>MKSVITTTISAADAAGRYPSTSDLQSVQGNIQRAAARLEAAEKLGSNH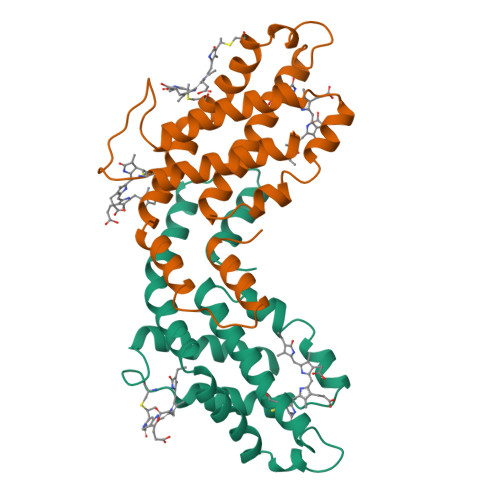EAVVKEAGDACFSKYGYNKNPGEAGENQEKINKCYRDIDHYMRLINYTLVVGGTGPLDEWGIAGAREVYRTLNLPSAAYIAAFVFTRDRLCIPRDMSAQAGVEFCTALDYLINSLS[2x];>[2x]MLDAFSRVVVNSDSKAAYVSGSDLQALKTFINDGNKRLDAVNYIVSNSSCIVSDAISGMICENPGLITPGGNCYTNRRMAACLRDGEIILRYVSYALLAGDASVLEDRCLNGLKETYIALGVPTNSTVRAVSIMKAAAVCFISNTASQRKVEVIEGDCSALASEVASYCDRVVAAVS> MANKEEIIAKAKEAITDFDDELAEEVANEALAAGIDPVELIEKGFT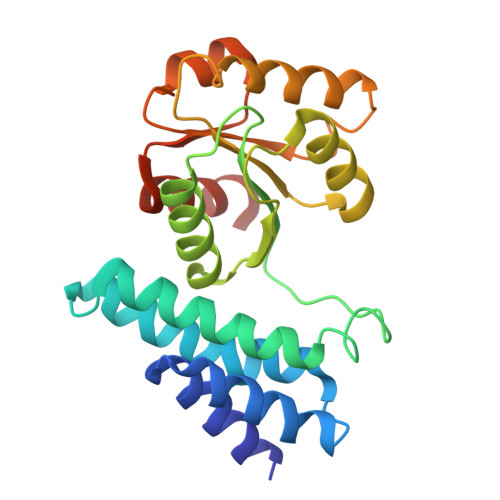AGMEEVGEKFGQGELFLPHVLAAAEAMNSGIKVITPEMEKRKSQTKSLGTVAIGTIEGDIHSIGKDIVASMLNIAGFKVVDLGRDVPINTFVEKVKELKPQVVASSALMTTTMVNQIQIEEQLKEAGVRDQVKTMVGGAPVTQDWADKIGADIYGESANDAVAKVKAALNVGGHHHHH> SNNWAVAPGRTAT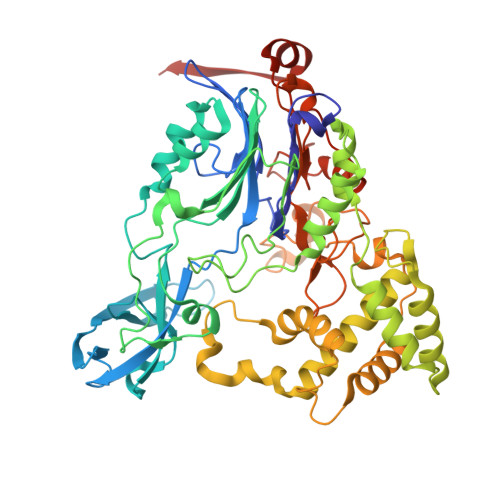GRPILAGDPHRVFEIPGFYAQHHLACDRFDMIGLTVPGVPGFPHFAHNGKVAYCVTHAFMDIHDLYLEQFAGEGRTARFGNDFEPVAWSRDRIAVRGGADREFDIVETRHGPVIAGDPRDGAALTLRSVQFAETDLSFDCLTRMPGASTVAQLYDATRGWGLIDHNLVAGDVAGSIGHLVRARVPSRPRENGWLPVPGWSGEHEWRGWIPHEAMPRVIDPPGGIIVTANNRVVADDHPDYLCTDCHPPYRAERIMKRLVANPAFAVDDAAAIHADTLSPHVGLLRRRLEALGARDDSAAEGLRQMLVAWDGRMDAASEVASAYNAFRRALTRLVTDRSGLEQAISHPFAAVAPGVSPQGQVWWAVPTLLRDDDAGMLKGWSWDQALSEALSVASQNLTGRSWGEEHRPRFTHPLATQFPAWAGLLNPASRPIGGDGDTVLANGLVPSAGPQATYGALSRYVFDVGNWDNSRWVVFHGASGHPASAHYADQNAPWSDCAMVPMLYSWDRIAAEAVTSQELVPALEHHHHHH>[2x]GVQADYSRAEALAAW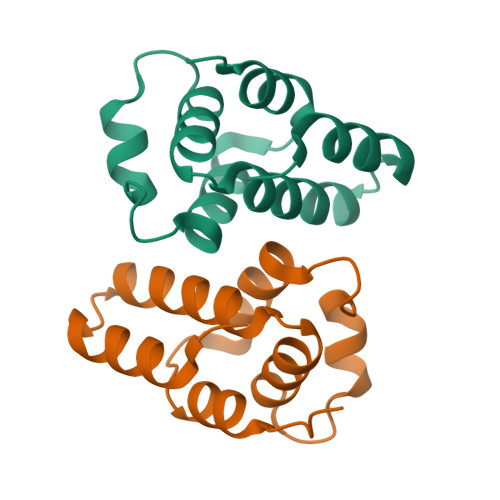TRLSDEFIGNCYVSVRPRHAPAWEVVVASAAGSLRLEAFKRAHDHDFLDRLAVAIGNWEQKAQRPDHEIAQMLDQVGDYG> SVPIQCTD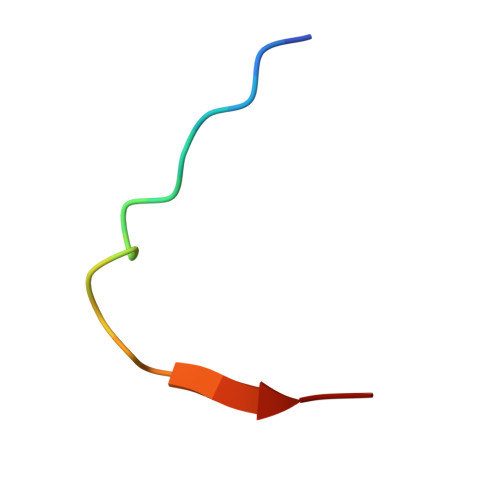KTDKQEALFK> GPLGSMASFKLATDLPEWKKLEETYKSVGEKFSVRDAFAKDPKRFEEFSWIYKNYDDSKILFDFSKNLVNKEIL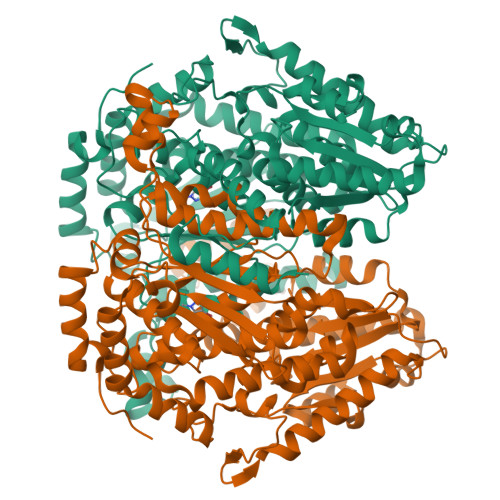DQLVTLAKEAGVEKLRDAMFAGDHINTTEDRAVYHVALRNRALRKMPVDGKDTAQEVDDVLKHMKEFSDSIRDGSWTGYTGKSITDVVNIGIGGSDLGPVMVTEALKAYSKPGLNVHFISNIDGTHTAETLKNLNPETTLFLIASKTFTTAETITNATSAKNWFLATAKDSKHIAKHFAALSTNEKEVVAFGIDAKNMFGFESWVGGRYSVWSAIGLSVAIYIGFENFNDFLKGAEAMDQHFLTTPLENNIPVIGGLLSVWYNNFFGAQTHLVVPFDQYLHRFPAYLQQLSMESNGKSVTRANVFTNYQTGTILFGEPATNAQHSFFQLVHQGTKLIPADFILAAQSHNPIEKNLHQRMLASNFFAQSEALMVGKDEAKVKAEGATGGLVPHKEFSGNRPTTSILAQKITPATLGSLIAYYEHLTFTEGAIWNINSFDQWGVELGKVLAKVIGKELDDKKAVATHDASTNGLINQFKEWEE> FPTIPLSRLFDNAMLRAHRLHQLAFDTYQEFEEAYIPKEQKYSFLQNPQTSLCFSESIPTPSNREETQQKSNLELLRISLLLIQSWLEPVQFLRSVFANS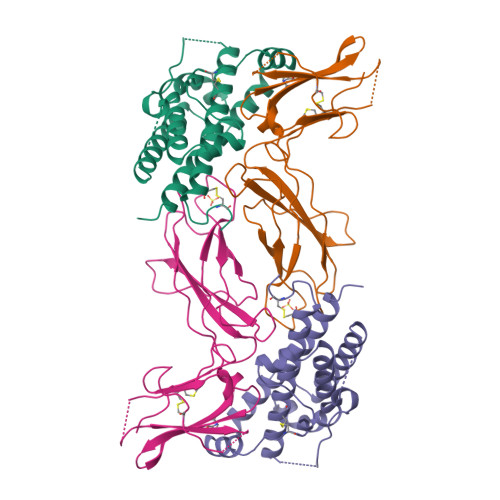LVYGASDSNVYDLLKDLEERIQTLMGRLTDGSPRTGQIFKQTYSKFDTNSHNDDALLKNYGLLYCFRRDMTYVATYLRIVQCRSVEGSCGF;> FSGSEATAAILSRAPWSLQSVNPGLKTNSSGEPKFTKCRSPERETFSCHWTDEVHHGTKNEGPIQLFYTRRNTQEWTQEWKECPDYVSAGENSCYFNSSFTSIAIPYCIKLTSNGGTVDEKCFSVDEIVQPDPPIALNWTLLNVSLTGIHADIQVRWEAPRNADIQKGWMVLEYELQYKEVNETKWKMMDPILTTSVPVYSLKVDKEYEVRVRSKQRNSGNYGEFSEVLYVTLPQM GmhA is conserved in many Gram‐negative and some Gram‐positive bacteria and is responsible for catalyzing isomerization of the D‐sedoheptulose 7‐phosphate into D‐glycero‐α,β‐D‐manno‐heptose‐7‐phosphate, which is the first and common step for parallel biosynthetic pathways leading to generation of GDP‐D‐glycero‐α‐D‐manno‐heptose (D,D‐heptose) and ADP‐L‐glycero‐β‐D‐manno‐heptose [L,D‐heptose; reviewed in Ref: (Valvano et al., 2002)]. GmhAGC consists of 197 amino acids with residues 37–197 comprising a sugar isomerase domain (SIS) that is shared between all ketose/aldose isomerases (Golinelli‐Pimpaneau, Le Goffic, & Badet, 1989). At the amino acid level, GmhAGC shows 43–57% identity with crystallized orthologous proteins and contains the key conserved residues observed in all GmhA homologs, including three serine residues and a threonine that presumably interact with the phosphate group of sedoheptulose 7‐phosphate or D‐glycero‐D‐manno‐heptose 7‐phosphate (Harmer, 2010; Valvano et al., 2002). We demonstrated that GmhA homologs in Neisseria gonorrhoeae and N. meningitidis (hereafter called GmhAGC and GmhANM, respectively) were interchangeable proteins essential for lipooligosaccharide (LOS) synthesis, and their depletion had adverse effects on neisserial viability.

The untagged GmhAGC crystallized as a tetramer in the closed conformation with four zinc ions in the active site, supporting that this is most likely the catalytically active conformation of the enzyme. Four monomers of GmhAGC were present in the asymmetric unit. The tetrameric architecture is consistent with the results of size exclusion chromatography, and with the previously determined structures of GmhA homologs from other bacteria. The interface area of the GmhAGC tetramer is extensive and buries 14,160 Å2 of surface area as calculated by the PISA server. John Wiley & Sons, LtdEach monomer of GmhAGC is composed of a central five‐stranded parallel β‐sheet flanked by four α‐helices from each side. Residues 69–74 (chains A and B) and 69–75 (chains C and D) are disordered in the structure. These residues form a loop in the vicinity of the active site and could become ordered upon substrate binding. The zinc ions are coordinated by the side chains of residues H61, E65, and H183 of one monomer, and the side chain of Q175 of the neighboring monomer. Zinc ions were not added to any of the protein purification steps or crystallization buffers, yet similar to Burkholderia pseudomallei GmhA, GmhAGC held zinc ions in the active site, providing further support that GmhA is a metalloenzyme. Zinc binding likely drives the “closed” conformation of GmhAGC, which was also observed in structures of B. pseudomallei, P. aeruginosa, and V. cholerae GmhA, thus providing further support that the “closed” conformation is catalytically relevant.

>GAMATLQERVAAHFAESIRAKQEAEKILVEPTVQAAELMLQCLMNDGKILACGNGGSAADAQHFAAEMTGRFEKERMELAAVALTTDTSALTAIGNDYGFDHVFSKQVRALGRAGDVLVGISTSGNSANVIEAVKAAHERDMHVIALTGRDGGKIAAMLKDTDVLLNVPHPRTARIQENHILLIHAMCDCIDSVLLEGMKLAAA[4x]>GSHSWQARLQDENASLAHQAHHDSLTSLPNRAFFEGRLSRALRDANEHREQLAVLFIDSDRFKEINDRLGHAAGDTVLVNIAMRIRGQLRESDLVARLGGDEFAVLLAPLASGADALRIADNIIASMQAPIRLSDGSTVSTSLTIGIALYPEHADTPAAL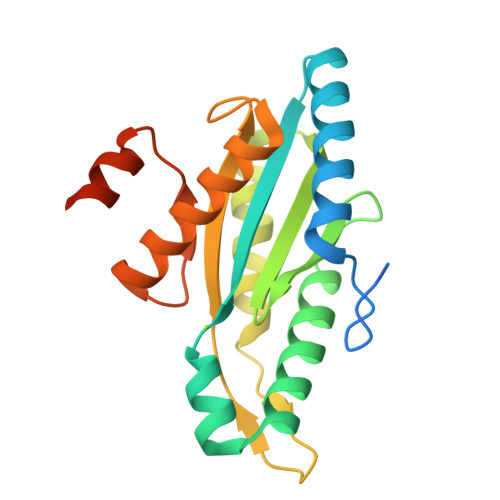LHDADMAMYIAKRQARGSRRLAELNDPRILQEEKEIDSATPEAPPK[3x]> GPLGSENDLGITAVALYDYQAAGDDEISFDPDDIITNIEMIDDGWWRGVCKGRY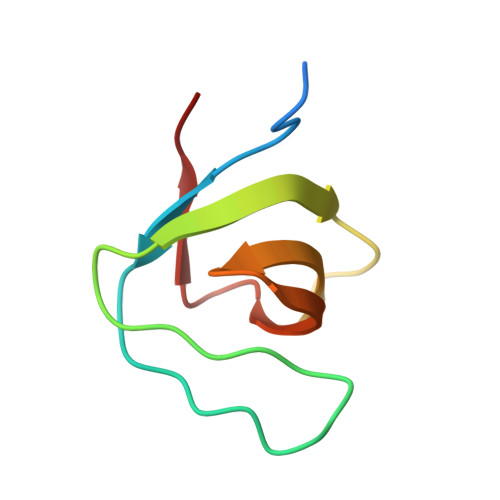GLFPANYVELRQ> HPETLVKVKDAEDQLGARVGYIELDLNSGKILESFRPEERFPMMSTFKVLLCGAVLSRVDAGQEQLGRRIHYSQNDLVEYSPVTEKHLTDGMTVRELCSAAITMSDATAANLLLTTIGGPKELTAFLHNMGDHVTRLDRWEPELNEAIPN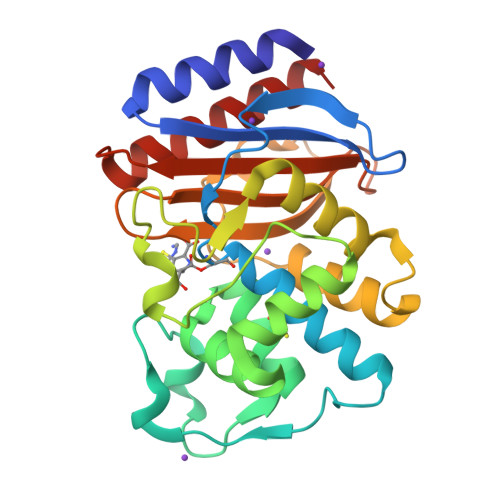DERDTTMPAAMATTLRKLLTGELLTLASRQQLIDWMEADKVAGPLLRSALPAGWFIADKSGAGERGSRGIIAALGPDGKPSRIVVIYTTGSQATMDERNRQIAEIGASLIKHW>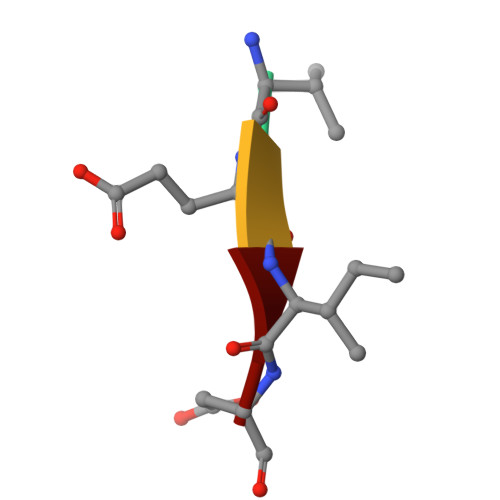 VEID> MKIAVLSRNPRLYSTR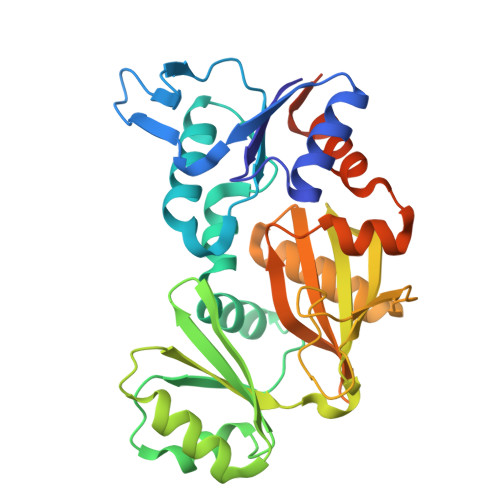RLVEAGRERGHEMVVIDTLRAYMNIASHKPQIHYRGQPLEGFDAVIPRIGASVTFYGCAVLRQFEMMGVFPLNESVAIARSRDKLRSLQLLSRKGIGLPVTGFAHSPDDVPDLIEMVGGAPLVIKLLEGTQGIGVVLCETEKAAESVLEAFMGLKHNIMVQEYIKEAGGADIRCFVVGDKVIASMKRQAAPGEFRSNLHRGGSASLIKITPEERMTAIRAARVMGLNVAGVDILRSNHGPLVMEVNSSPGLEGIESTTGKDIAGIIIQYLEKNGGPHLARTKGKGKLAAALEHHHHHH>MGHHHHHHLESTSLYKKSSSTPPRGVTVVNNFDCKRYLGTWYEIARFDHRFERGLEKVTATYSLRDDGGLNVINKGYNPDRGMWQQSEGKAYFTGAPTRAALKVSFF[3x];>[3x]MGPFYGGYNVIALDREYRHALVCGPDRDYLWILSRTPTISDEVKQEMLAVATREGFDVSKFIWVQQPGS

In our previous work, using a combination of computational and in vitro screenings we created a panel of FAPs from bacterial lipocalin Blc (named DiBs) capable of recovering the fluorescence of synthetic analogs of green and red fluorescent proteins’ chromophores. The lipocalin fold contains a single eight-stranded continuously hydrogen-bonded antiparallel β-barrel complemented by an α-helix. Fluorogen-activating proteins (FAPs) are a group of unrelated proteins capable of binding to non-protein ligands (fluorogens) and increase the fluorescence quantum yield and/or change spectral properties of these ligands. Here we report on DiB-splits, a self-assembling FAP split system which has been inspired by the domain-swapped structure of a full-length DiB protein.

To further confirm the recovery of the lipocalin fold by split DiBs, we crystalized the DiB2-split protein. Crystals diffracted to approximately 2 Å and contained three “split” molecules per asymmetric unit. According to size-exclusion chromatography conducted during purification routine of split proteins there were no signs of oligomerization of any kind. The main difference between superimposed monomers from the asymmetric unit is observed in the termini of the two β-strands adjacent to the cleavage site. These residues are involved in crystal packing interactions in the DiB2-split crystal. The residues of the hinge loop and two adjacent β-strands are also responsible for the main difference between wtBlc and DiB2-split monomers. The observed differences between structures might be partially caused by releasing the tension in the fold through polypeptide chain cleavage. Despite these minor structural deviations, the overall lipocalin fold as well as specific intramolecular β-barrel stabilizing interactions, which became intermolecular interactions after the splitting, are well preserved in the DiB2-split structure. This confirms that the split system is capable of spontaneous correct self-assembly to form the functional protein.>GSRRYDVFPSFRGEDVRDSFLSHLLKELRGKAITFID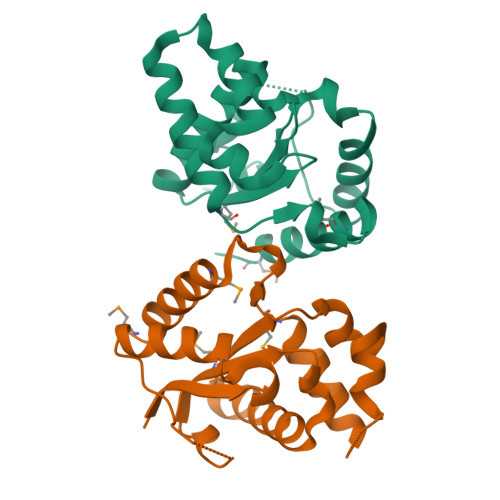DEIERSRSIGPELLSAIKESRIAIVIFSKNYASSTWCLNELVEIHKCYTNLNQMVIPIFFHVDASEVKKQTGEFGKVFEETCKAKSEDEKQSWKQALAAVAVMAGYDLRKWPSEAAMIEELAEDVLRKTMTPSDDFG[2x]>[4x]MGSSHHHHHHSQDHENLYFQGSMGLEKGFTHPTDRVVRLKNMILHAKPYVESERAVLATEAYKENEQLPAIMRRAKVVEKIFNELPVTIRPDELIVGAVTINPRSTEICPEFSYDWVEKEFDTMAHRVADPFIIEKKTADELHQAFKYWPGKTTSSLAASYMSEGTKESMSNGVFTVGNYFFGGIGHVSVDYGKVLKIGFRGIIDEVTRAL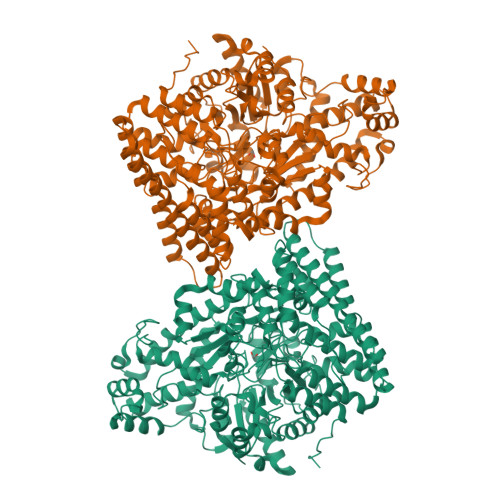ENLDRSTSDYIKKEQFYNAVILSYQAAINFAHRYAQEASRLAREERDPTRQRELEQIASNCTRVPEYGATTFWEACQTFWFIQSMLQIESSGHSISPGRFDQYMYPYLAADTAISSEFAQELVDCCWIKLNDINKTRDEISAQAFAGYAVFQNLCVGGQTEDGRDATNPLTYMCMEATAHVRLPQPSFSIRVWQGTPDEFLYRACELVRLGLGVPAMYNDEVIIPALQNRGVSLHDARDYCIIGCVEPQAPHRTEGWHDAAFFNVAKVLEITLNNGRSGNKQLGPMTGEMTQYAGMDDFYAAFKKQMAHFVHQLVEACNSVDIAHGERCPLPFLSALVDDCIGRGKSLQEGGAIYNFTGPQAFGIADTGDSVYAIQKQVFEDRRLTLQELKGALDANFGYRSGNPRYEEIRHILENSPCFGNDIDDVDLVARQCALIYCQEVEKYTNPRGGRFQAGIYPVSANVLFGKDVSALPDGRLAKEPLADGVSPRQGKDTLGPTAAANSVAKLDHFIASNGTLYNQKFLPSSLAGEKGLRNFGGLVRNYFDKKGMHVQFNVIDRNTLLEAQKNPQQHQDLVVRVAGYSAQFVVLAKEVQDDIISRTEQQF>GGAGCCCC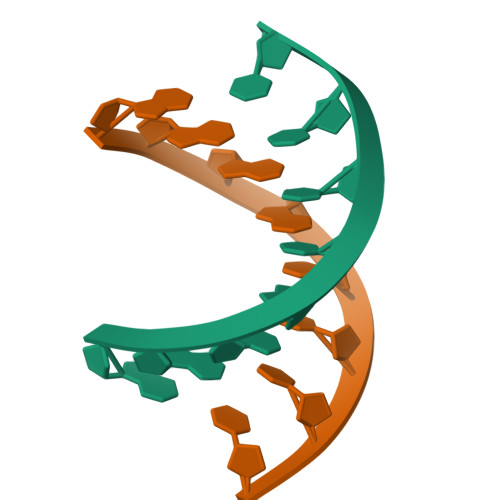[2x]>SNAAGTTVKKETAKKSASKTPAPKKKATLKVSKNHINYTMDKRGKKPEGMVIHNDAGRSSGQQYENSLANAGYARYANGIAHYYGSEGYVWEAIDAKNQIAWHTGDGTGANSGNFRFAGIEVCQSMSASDAQFLKNEQAVFQFTAEKFKEWGLTPNRKTVRLHMEFVPTACPHRSMVLHTGFNPVTQGRPSQAIMNKLKDYFIKQIKNYMDKGTSSSTVVKDGKTSSASTPATRPVTGSWKK[4x]

The staphylococcal phage lysin LysGH15 demonstrates great potential against methicillin-resistant Staphylococcus aureus (MRSA). Lysin (also known as endolysin) is a cell wall hydrolase that is synthesized at the end of the phage lytic life cycle and is involved in cell lysis and the release of progeny particles from host cells. LysGH15 shares very high sequence identity with other lysins of class III staphylococcal phages, such as LysK, phi11, and MV-L. Moreover, these lysins possess a modular structure containing an N-terminal CHAP domain (cysteine, histidine-dependent amidohydrolases/peptidases), a central amidase-2 domain (N-acetylmuramoyl-L-alanine amidase), and a C-terminal SH3b domain (the SH3 bacterial binding domain, which typically contains 60–70 residues and is homologous to eukaryotic SH3 proteins). To elucidate the molecular mechanism, we determined the structures of three individual LysGH15 domains using X-ray crystallography or nuclear magnetic resonance (NMR).

The structure of the amidase-2 domain (residues 165–403) was determined at 2.27 Å resolution. PSI-BLAST analysis using the National Center for Biotechnology Information (NCBI) database reveals that the amidase-2 domain contains a conserved zinc-binding site. Structure-based mutagenesis also confirms that E282 and the zinc ion play an important role in maintaining the lytic activity of the amidase-2 domain. Although the sequences of the LysGH15 amidase-2 domain and AmiD are divergent, they exhibit homologous structures and share conserved active site residues. In AmiD, E104 (E282 in the LysGH15 amidase-2) and a zinc ion activate the water that is bound to the zinc ion, which favors the nucleophilic attack of the amide bond; the tetrahedral intermediate is stabilized by K159 (this site is occupied by T330 in the LysGH15 amidase-2 domain). Mutational analysis demonstrates that E282 and T330 are critical for the activity of the LysGH15 amidase-2 domain. Thus, the amidase-2 domain of LysGH15 most likely possesses a similar catalytic mechanism as AmiD. Here, we find that the amidase-2 domain of LysGH15 from phage (virus) also contains this conserved residue (i.e., N275) at a corresponding position as other amidase members. Nevertheless, the LysGH15 amidase-2 domain is not entirely silent but additionally exhibits the ability to enhance the lytic activity of the CHAP domain. Therefore, the amidase-2 domain may cleave specialized substrates of the peptidoglycan, such as the bond between N-acetylmuramoyl-L-alanine.2'-tert-butyl-1-(2H-indazol-5-ylcarbonyl)-2'H-spiro[piperidine-4,5'-pyrano[3,2-c]pyrazol]-7'(6'H)-one | C22 H25 N5 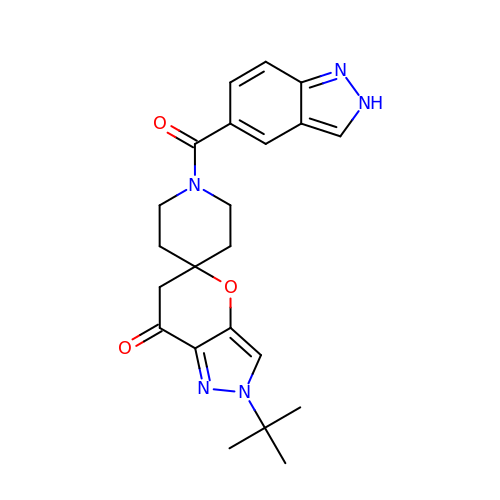O3 | MDLAYXJCVDNKAB-UHFFFAOYSA-N>[6x]VEQDPFEIAVKQLERAAQYMDISEEALEFLKRPQRIVEVSIPVEMDDGSVKVFTGFRVQYNWARGPTKGGIRWHPEETLSTVKALAAWMTWKTAVM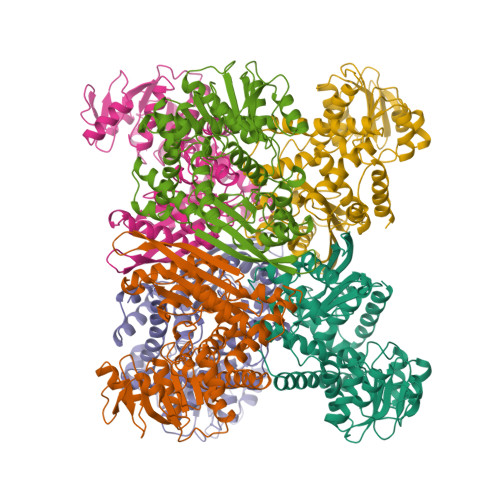DLPYGGGKGGVICNPKEMSDREKERLARGYVRAIYDVISPYTDIPAPDVYTNPQIMAWMMDEYETISRRKDPSFGVITGKPPSVGGIVARMDATARGASYTVREAAKALGMDLKGKTIAIQGYGNAGYYMAKIMSEEYGMKVVAVSDTKGGIYNPDGLNADEVLAWKKKTGSVKDFPGATNITNEELLELEVDVLAPSAIEEVITKKNADNIKAKIVAELANGPTTPEADEILYEKGILIIPDFLCNAGGVTVSYFEWVQNITGDYWTVEETRAKLDKKMTKAFWDVYNTHKEKNINMRDAAYVVAVSRVYQAMKDRGWIKK> QEGDPEAGAKAFNQCQTCHVIVDDSGTTIAGRNAKTGPNLYGVV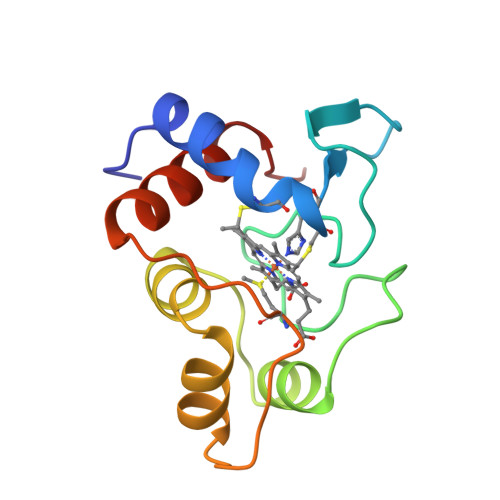GRTAGTQADFKGYGEGMKEAGAKGLAWDEEHFVQYVQDPTKFLKEYTGDAKAKGKMTFKLKKEADAHNIWAYLQQVAVRP>GSHMDGTEKWRFKTGKAIEASPVIGEDGTIYVGSNDGHLYAINPDGTEKWRFKTGKAIEASPVIGEDGTIYVGSNDGHLYAINPDGTEKWRFKTGKAIEASPVIGEDGTIYVGSNDGHLYAINPDGTEKWRFKTGKAIEASPVIGED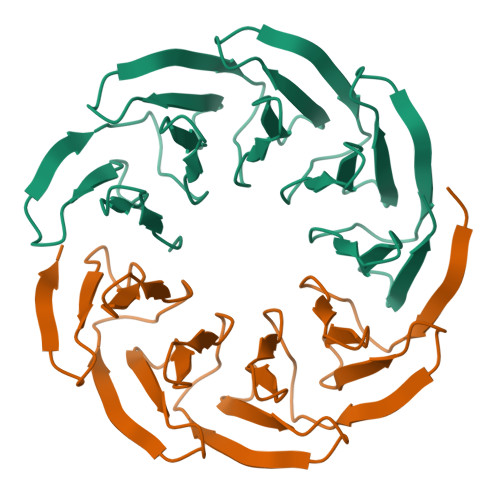GTIYVGSNDGHLYAINPDGTEKWRFKTGKAIEASPVIGEDGTIYVGSNDGHLYAINP[2x]> HMVPACPPPNPHQVEQLQDFVSQSQRLFVMTGAGISTESGIPDYRSEGVGLYSRTERRPIQHSEFVQSQAARRRYWARNFVGWPSFSSHEPNSAHVNLCKWERAGRLHWLVTQNVDALHTKAGQCRLSELHGCTHRVICLGCQTVTKRSELQERFLNLNPSWNEQAHGLAPDGDVFLTDEQVSDFQVPACTKCGGILKPQVTFFGDTVNRGFVFSIYEQMKQADAMLIVGSSLQVYSGYRFALNAKELHLPIAILNIGPTRADHLAKVKVSARCGDVLPHILLQDQ

Among the protein Lys deacetylases, sirtuins form the evolutionary defined class III. Sirtuins are increasingly recognized as deacylases with isoform-specific acyl selectivities, catalyzing removal of acylations emerging as posttranslational protein modifications, such as succinylation or crotonylation. The sirtuin core comprises a Rossmann-fold subdomain and a smaller Zn2+-binding module. The isoform differences in preferred substrate acyls are caused by binding of the acyl moiety to an active site channel with isoform-specific features.

xSirt4 yielded well diffracting crystals in presence of ADP-ribose (ADPr). The xSirt4 overall structure shows the typical sirtuin architecture with Rossmann-fold domain and smaller Zn2+-binding module, with the active-site located in between them and harboring the nucleotide that is well defined by electron density. The six-stranded β-sheet of the Rossmann-fold domain provides a docking patch for the nucleotide, orienting the reacting ribose close to the conserved catalytic sirtuin residue His160 (numbering refers to xSirt4 if not stated otherwise). Due to the occupied nucleotide binding site, the cofactor-binding loop between α2 and α3 is in the “closed” conformation, positioning the conserved Phe/Tyr (Tyr73) on top of the ADPr ribose. Comparing the Sirt4 structure to other sirtuin isoforms reveals as most striking difference an extended, ~12 residues Sirt4 loop in the Zn2+-binding module, between α8 and α9 (residues 195–206). The loop is oriented deep into the catalytic core and contributes to the active site lining. Another unusual feature of the Sirt4 catalytic core is a channel that branches off from the acyl-Lys binding tunnel and leads to the protein surface. It is lined by residues from α4 and the preceding loop (86-ArgArgProIle, Glu93), α5 (Ala100, 103-ArgTyr, Arg107), and Ala199/Asp203 from the Sirt4-loop. The Sirt4 channel has a small positively charged patch at the outer entrance but is generally rather hydrophobic, and we speculate that it contributes to accommodation of longer substrate acyls. Modeling a Sirt4/lipoyl-Lys complex indeed places the distal lipoyl end into the bottom of the channel, supporting an acyl binding function and rationalizing Sirt4’s delipoylation activity.> MKAWVLKRLGGPLELVDLPEPEAEEGEVVLRVEAVGLNFADHLMRLGAYLTRLHPPFIPGMEVVGVVEGRRYAALVPQGGLAERVAVPKGALLPL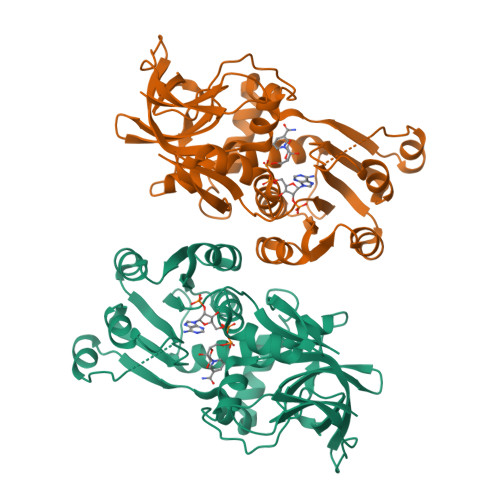PEGLSPEEAAAFPVSFLTAYLALKRAQARPGEKVLVQAAAGALGTAAVQVARAMGLRVLAAASRPEKLALPLALGAEEAATYAEVPERAKAWGGLDLVLEVRGKEVEESLGLLAHGGRLVYIGAAEGEVAPIPPLRLMRRNLAVLGFWLTPLLREGALVEEALGFLLPRLGRELRPVVGPVFPFAEAEAAFRALLDRGHTGKVVVRL>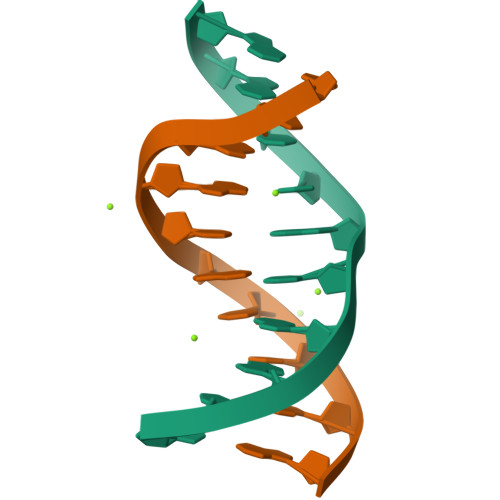[4x]CCGGTACCGG5-methyl-6-(naphthalen-1-ylsulfanyl)thieno[2,3-d]pyrimidine-2,4-diamine 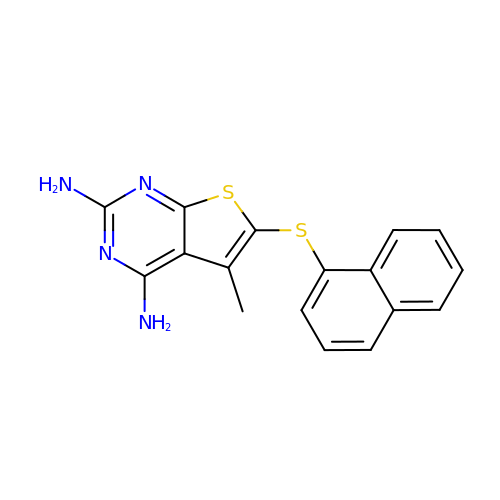| C17 H14 N4 S2 | DSWPJTXRDPNDRO-UHFFFAOYSA-N> MTNPFDNEDGSFLVLVNGEGQHSLWPAFAEVPD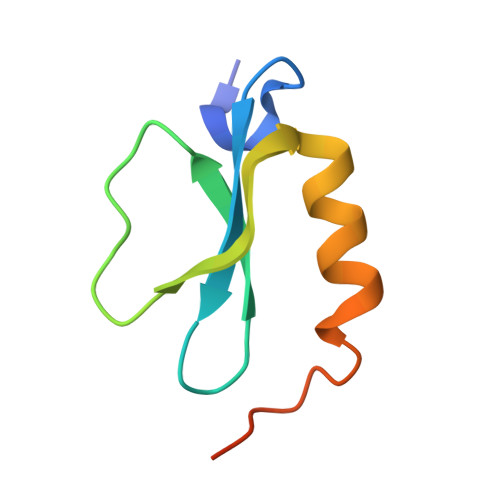GWTGVHGPASRQDCLGYVEQNWTDLRPKSLISQISD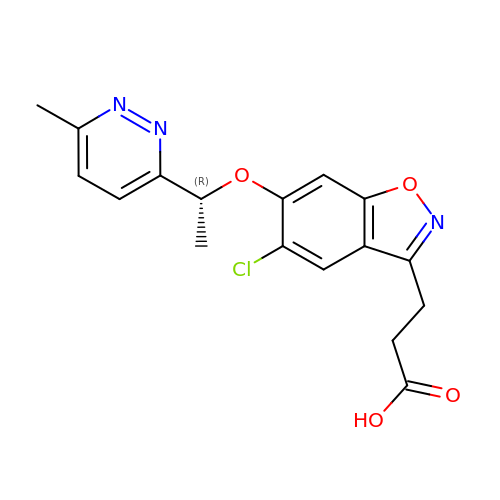3-[5-chloranyl-6-[(1~{R})-1-(6-methylpyridazin-3-yl)ethoxy]-1,2-benzoxazol-3-yl]propanoic acid | C17 H16 Cl N3 O4 | YWASLAPMFGBZQP-SNVBAGLBSA-N>MEVSRISYEDIGGLSEQLGKIREMIELPLKHPELFERLGITPPKGVILYGPPGTGKTLIARAVANESGANFLSINGPEIMSKYYGQSEQKLREIFSKAEETAPSIIFIDEIDSIAPKREEVQGEVERRVVAQLLTL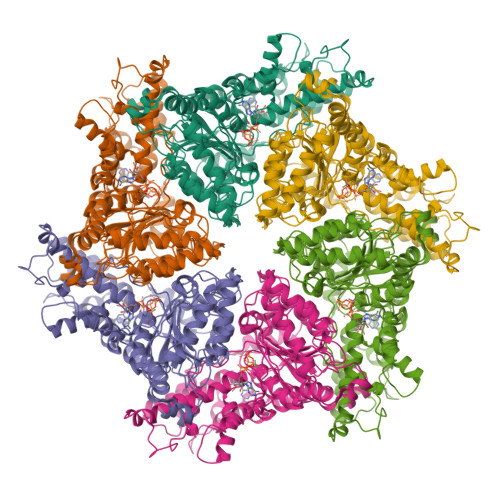MDGMKERGHVIVIGATNRIDAIDPALRRPGRFDREIEIGVPDRNGRKEILMIHTRNMPLGMSEEEKNKFLEEMADYTYGFVGADLAALVRESAMNALRRYLPEIDLDKPIPTEILEKMVVTEDDFKNALKSIEPSSLREVMVEVPNVHWDDIGGLEDVKREIKETVELPLLKPDVFKRLGIRPSKGFLLYGPPGVGKTLLAKAVATESNANFISIKGPEVLSKWVGESEKAIREIFKKAKQVAPAIVFLDEIDSIAPRRGTTSDSGVTERIVNQLLTSLDGIEVMNGVVVIGATNRPDIMDPALLRAGRFDKLIYIPPPDKEARLSILKVHTKNMPLAPDVDLNDIAQRTEGYVGADLENLCREAGMNAYRENPDATSVSQKNFLDALKTIRPSVDEEVIKFYRTLSETMSKSVSERRKQLQDQGLYL[6x]> MGLNFFRKAAPEVRTEPVAERKASVTGRIVAMASGAGRPVWGPRDTVSLMRTGFAGNPVGFRSVKLIAEATAAVPLICQDAERRYEIHPVLDLLRRPNAGQGRAELFEALIGQILLSGNGYLEAVCPEPGVPRELH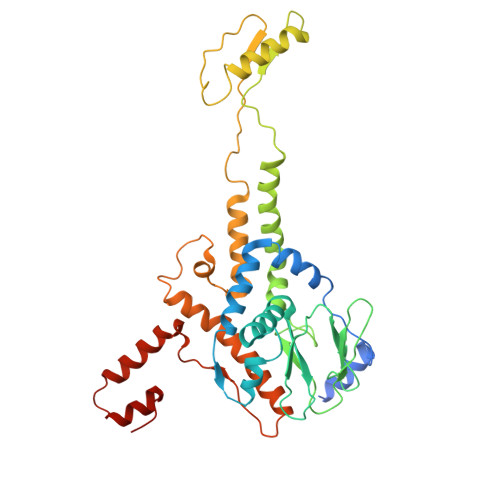VLRSDRMAVVPGADGWPVGYDYTVGGRKHRFDMTGHPDPICHIKSFHPTDDHYGLSPMQAAAVALDVHNAASAWSKALLDNAARPSGAIIYKGADGQGVLAPEQYERLIFEMETHHQGARNAGRPMLLEGGLDWKPMGFSPSDMEFHETKAAAAREIALAFGVPPMLIGIPGDATYANYAEANRAFYRLTVLPLLTRVSAALAWWLSGYLGAQIELKPDLDQVPALAVERDQLWARIGAAGFLSNSEKRVLLGLPPTAEG>[2x]MWRYPRNADQTFWAFRTCQRQSEGAKSLREWYRWNLPNDEDTHCY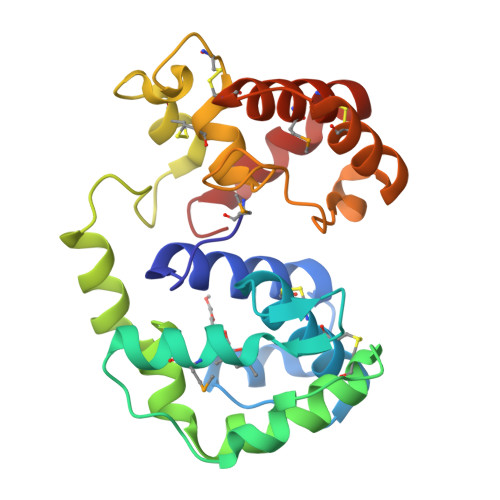VKCVWLHLGLYNEQNKSLRVDRIMEQFNSRSVAIPGGINTISGPTDGTCKDIYDKTINFFNNNVNDLRTAFYGIKKLSDEWFTQNSNTKPKGTKISDFCNAENREKGGADCQHACSAYYYRLVDEDNEPIHFRNLNILGITDEQFASCVKASKNKQGCKVADTMYNCVEKHNSQALKILDNQSPTY>ENTLTVKMNDALSSGTGENIGEITVSETPYGLLFTPHLNGLTPGIHGFHVHTNPSCMPGMKDGKEVPALMAGGHLDPEKTGKHLGPYNDKGHLGDLPGLVVNADGTATYPLLAPRLKSL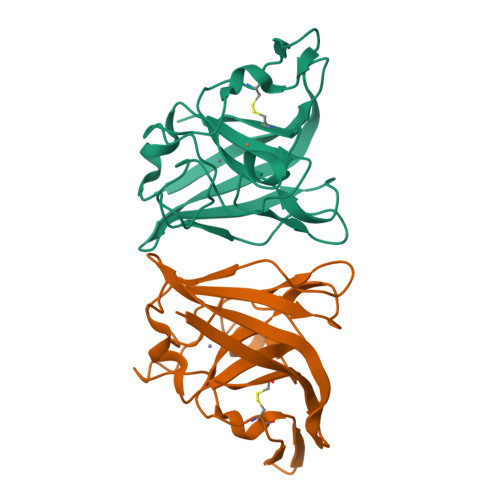SELKGHSLMIHKGGDNYSDKPAPLGGGGARFACGVIEKLEHHHHHH[2x]> MSGKAQQQSRLKELIARGREQGYLTYAEVNDHLPEDISDPEQVEDIIRMINDMGINVFETAPDADALLLAEADTDEAAAEEAAAALAAVESDIGRTTDPVRMYMREMGTVELLTREGEIEIAKRIEEGIREVMSAIAQFPGTVDSILADYNRIVAEGGRLSDVLSGYIDPDDGSLPAEEVEPVNLKDDSADSKEKDDEEEESDDSSDSDDEGDGGPDPEEARLRFTAVSEQLDKAKKALKKHGRGSKQATAELTGLAELFMPIKLVPKQFDALVARVRSALEGVRAQERAIMQLCVRDARMPRADFLRLFPNHETDEKWVDSVLKSKPKYAEAIERLRDDILRNQQKLAALESEVELTVAEIKEINRAMSIGEAKARRAKKEMVEANLRLVISIAKKYTNRGLQFLDLIQEGNIGLMKAVDKFEYRRGYKFSTYATWWIRQAITRSIADQARTIRIPVHMIETINKLNRISRQMLQEMGREPTPEELGERMDMPEDKIRKVLKIAKEPISMETPIGDDEDSHLGDF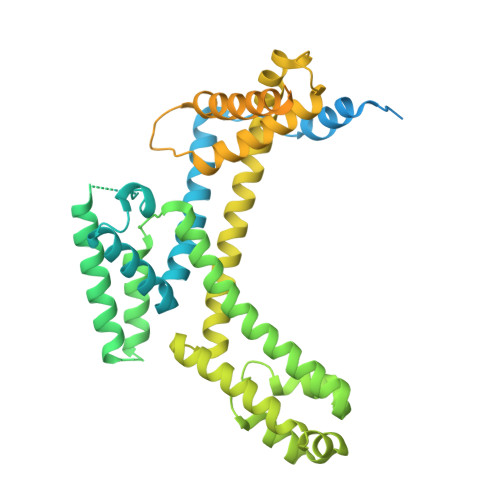IEDSTMQSPIEMATSESLKESTREVLAGLTAREAKVLRMRFGIDMNTDHTLEEVGKQFDVTRERIRQIEAKALRKLRHPSRSEHLRSFLDE> GAEFDLDQGGEALAPRQVLDLEDLVFTQGSHFMANKRCQLPDGSFRRQRKGYEEVHVPALKPKPFGSEEQLLPVEKLPKYAQAGFEGFKTLNRIQSKLYRAALETDENLLLCAPTGAGKTNVALMCMLREIGKHINMDGTINVDDFKIIYIAPMRSLVQEMVGSFGKRLATYGITVAELTGDHQLCKEEISATQIIVCTPEKWDIITRKGGERTYTQLVRLIILDEIHLLHDDRGPVLEALVARAIRNIEMTQEDVRLIGLSATLPNYEDVATFLRVDPAKGLFYFDNSFRPVPLEQTYVGITEKKAIKRFQIMNEIVYEKIMEHAGKNQVLVFVHSRKETGKTARAIRDMCLEKDTLGLFLREGSASTEVLRTEAEQCKNLELKDLLPYGFAIHHAGMTRVDRTLVEDLFADKHIQVLVSTATLAWGVNLPAHTVIIKGTQVYSPEKGRWTELGALDILQMLGRAGRPQYDTKGEGILITSHGELQYYLSLLNQQLPIESQMVSKLPDMLNAEIVLGNVQNAKDAVNWLGYAYLYIRMLRSPTLYGISHDDLKGDPLLDQRRLDLVHTAALMLDKNNLVKYDKKTGNFQVTELGRIASHYYITNDTVQTYNQLLKPTLSEIELFRVFSLSSEFKNITVREEEKLELQKLLERVPIPVKESIEEPSAKINVLLQAFISQLKLEGFALMADMVYVTQSAGRLMRAIFEIVLNRGWAQLTDKTLNLCKMIDKRMWQSMCPLRQFRKLPEEVVKKIEKKNFPFERLYDLNHNEIGELIRMPKMGKTIHKYVHLFPKLELSVHLQPITRSTLKVELTITPDFQWDEKVHGSSEAFWILVEDVDSEVILHHEYFLLKAKYAQDEHLITFFVPVFEPLPPQYFIRVVSDRWLSCETQLPVSFRHLILPEKYPPPTELLDLQPLPVSALRNSAFESLYQDKFPFFNPIQTQVFNTVYNSDDNVFVGAPTGSGKTICAEFAILRMLLQSSEGRCVYITPMEALAEQVYMDWYEKFQDRLNKKVVLLTGETSTDLKLLGKGNIIISTPEKWDILSRRWKQRKNVQNINLFVVDEVHLIGGENGPVLEVICSRMRYISSQIERPIRIVALSSSLSNAKDVAHWLGCSATSTFNFHPNVRPVPLELHIQGFNISHTQTRLLSMAKPVYHAITKHSPKKPVIVFVPSRKQTRLTAIDILTTCAADIQRQRFLHCTEKDLIPYLEKLSDSTLKETLLNGVGYLHEGLSPMERRLVEQLFSSGAIQVVVASRSLCWGMNVAAHLVIIMDTQYYNGKIHAYVDYPIYDVLQMVGHANRPLQDDEGRCVIMCQGSKKDFFKKFLYE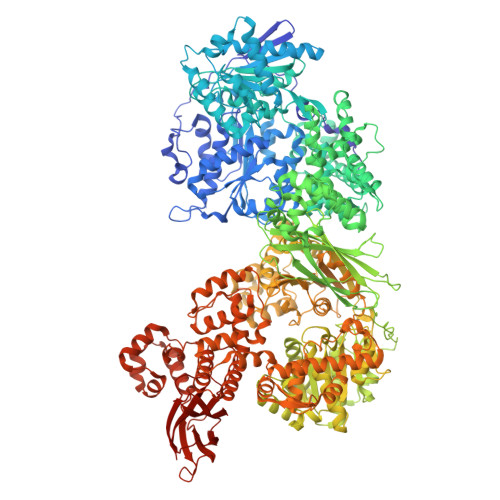PLPVESHLDHCMHDHFNAEIVTKTIENKQDAVDYLTWTFLYRRMTQNPNYYNLQGISHRHLSDHLSELVEQTLSDLEQSKCISIEDEMDVAPLNLGMIAAYYYINYTTIELFSMSLNAKTKVRGLIEIISNAAEYENIPIRHHEDNLLRQLAQKVPHKLNNPKFNDPHVKTNLLLQAHLSRMQLSAELQSDTEEILSKAIRLIQACVDVLSSNGWLSPALAAMELAQMVTQAMWSKDSYLKQLPHFTSEHIKRCTDKGVESVFDIMEMEDEERNALLQLTDSQIADVARFCNRYPNIELSYEVVDKDSIRSGGPVVVLVQLEREEEVTGPVIAPLFPQKREEGWWVVIGDAKSNSLISIKRLTLQQKAKVKLDFVAPATGAHNYTLYFMSDAYMGCDQEYKFSVDVKEA>SLELLEPPTQMRDLTASQLLDEITIGWNLGNTLDATTTSWLPNPTPAQSETAWGCPMTTKAMIDKVKEGGFNTVRVPVSWIDHTGSAPEYQIDEAWMNRVQEVVNYVIDNDMYCILNIHHENDWLIPTNAQKDSVNARLDAIWTQIATRFGSYDEHLIFEGMNQPRLVGDPNEWNGGNQEARQVINSYNQTFVNTVRATGGNNAIRCLMVPTYAASCSSTTVNDFVLPTDTVANKLIVDIHSYSPYNFALNTSGTSSFTQSDISQLQW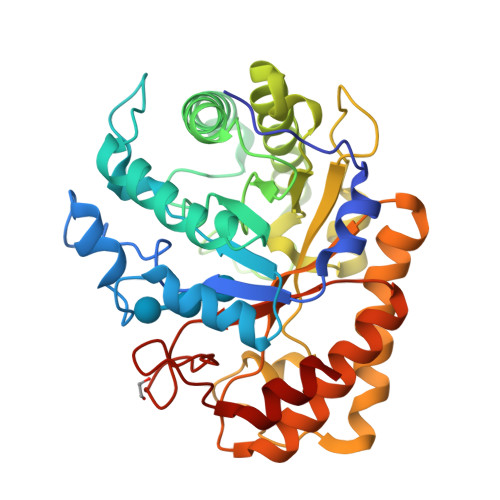TLQEIYNSFGAKGIPVIIGQFGALNKNNINGRVLWGENYLRIAKSYNIRCIWWDNNAFDTSGENFGLLNRGTLTWQYPELLEAMMK[4x]>SQLLNYIDGNFVTSASSFANINPVNGKLISDVFEADAKQVNEAVVAAQNALKGPWGKLSVQDRAALIHKIADGIQARFEEFVAAEVADTGRPVHQARTLDIPRAIANFRTFADLAKTSHTDLFEMSTSDGSGALNYTVRKPLGVIGVISPWNLPLLLFTWKVAPALACGNTVVAKPSEESPSSATLLAEVMHDAGVPPGVFNLIHGFGKDSAGEFLTQHPGISALTFTGESKTGSTIMKAVADGVKEVSFELGGKNAAVVFADADLDAAIEGVLRSSFTNSGQVCLCSERVYVHRSIFDEFVSGLKVEAERLVVGYPDQDGVNMGPLISHGHRDKVLSYYRLAVDEGATVVTGGGVPKFNDERDQGAYVQPTIWTGLSDKARCVTEEIFGPVCHISPFDDEDEVINRVNDSNYGLACAIWTTNLSRAHRVSRQIHVGLVWVNTWYLRDLRTPFGGVKLSGLGREGGRFSMDFYSDIANICIKI[4x]

One enzyme in particular, 2-aminomuconate-6-semialdehyde dehydrogenase (AMSDH), is responsible for oxidizing the unstable metabolic intermediate 2-aminomuconate-6-semialdehyde (2-AMS) to 2-aminomuconate (2-AM). On the basis of sequence alignment, AMSDH is a member of the hydroxymuconic-semialdehyde dehydrogenase (HMSDH) family under the aldehyde dehydrogenase (ALDH) superfamily. The complete AMSDH model includes four polypeptides per asymmetric unit describing one homotetramer. Each monomer of AMSDH contains three domains: a subunit interaction domain, a catalytic domain and an NAD+ binding domain.

Enzyme–NAD+ binary complex crystals were soaked in mother liquor containing 2-HMS for a range of time points from 5 min to more than 3 h before flash cooling in liquid nitrogen. In a crystal that was soaked for 40 min, an intermediate was trapped and refined to a resolution of 1.95 Å. In this structure, 2-HMS is observed in the 2Z, 4E isomer rather than the 2E, 4E isomer as seen in the substrate-bound ternary structure. Also, the substrate interacts with Arg120 and Arg464 with both of its carboxyl oxygens rather than one carboxyl oxygen and the 2-hydroxy oxygen as shown in the 2-HMS ternary complex structure. On E to Z isomerization, the carbon chain of the substrate extends, and the distance between its sixth carbon and Cys302’s sulfur is now at 1.8 Å, which is within covalent bond distance for a carbon–sulfur bond. Also, the continuous electron density between Cys302-SG and 2-HMS-C6 indicates the presence of a covalent bond. Another feature of this intermediate is that the nicotinamide ring of NAD+ has moved 4.6 Å away from the active site and adopted a bent conformation compared with the position in the binary or ternary complex structures. Thus, the coenzyme in this intermediate structure is likely to have been reduced to NADH and, as such, the structure is assigned as a thioacyl-enzyme–substrate adduct. Another notable change in the intermediate structure is the movement of the side chain of Glu268, which rotates 73° towards the active site. In the thioacyl intermediate structure, the electron density of Glu268 becomes very well defined again, but its side chain rotates 73° towards the bound substrate and seems to be in an ‘active’ position to abstract a proton from a deacylating water.>[2x]LIKHMRAEALFDFTGNSKLELNFKAG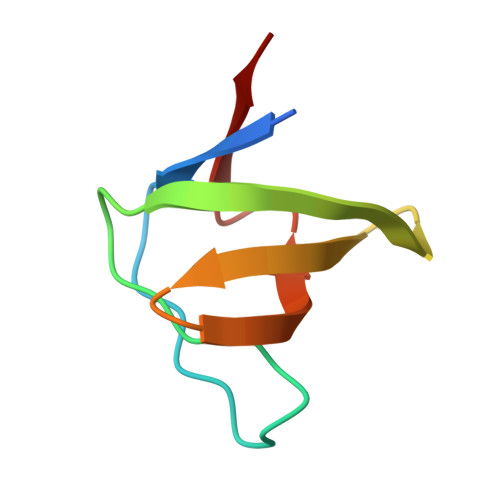DVIFLLSRINKDWLEGTVRGATGIFPLSFVKILK> SQLTKDEIEEVREVFDLFDFWDGRDGDVDAAKVGDLLRCLGMNPTEAQVHQHGGTKKMGEKAYKLEEILPIYEEMSSKDTGTAADEFMEAFKTFDREGQGLISSAEIRNVLKMLGERITEDQCNDIFTFCDIREDIDGNIKYEDLMKKVM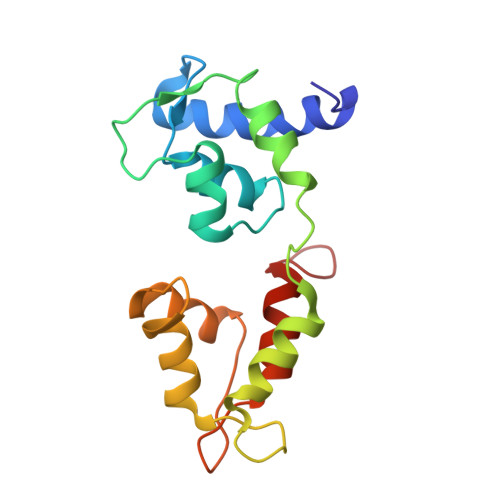AGPFPDKSD>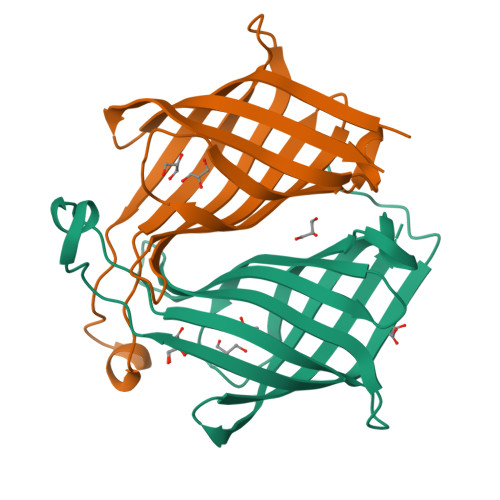GSHMSTVTTINLEDIKEIMHTTIRLGGKPESGEAAELPIFLGSSVEFEAELYDADGTQIGTAKGTSVIFAEADGTVMQIVSAFDDYTDGGRVTWSGAYTMFPTDEPKSVPAQGVSGRYRGLSGTRTFQLLERPDPGTSLVRSSLVLNG[2x]In this study, we present the cryo-EM structures of two thermostable multimeric enzymes that have different point-symmetry groups; namely SOR from Acidianus ambivalens and LS from Aquifex aeolicus. The reported cryo-EM structures of the two enzymes including their active sites correlate very well with the x-ray crystal structures. Due to their thermostability and relatively easy purification scheme, both SOR and LS can serve as a model for the catalytic and structural characterization of biocatalysts as well as a benchmark for cryo-EM sample preparation, optimization of the acquisition parameters and 3D reconstruction.

LS from the hyperthermophilic bacterium Aquifex aeolicus living in hot springs of up to 90°C is extremely thermostable with a 119.9°C melting temperature, which is ~27°C higher than that of the next thermostable LS from B. subtilis. LS catalyzes the formation of 6,7-dimethyl-8-ribityllumazine by condensation of 5-amino-6-(D-ribitylamino)uracil with 3,4-dihydroxy-2-butanone 4-phosphate. LS consists of 60 identical subunits that form a capsid of icosahedral 532 symmetry with an outer diameter of 154 Å and inner compartment diameter of 80 Å. Further processing and refinement resulted in a cryo-EM map at a global 2.33 Å resolution as depicted in the FSC plot. The RMSD of both structures is 0.174 Å for the 154 Cα atoms. The LS monomer is composed of a central four-stranded β-sheet flanked on one side by two α helices and on the other side by three α helices. There is a channel in the center of the pentamer formed by an α helix (α3) and its four symmetry-related neighbors, with a diameter of about 9 Å, where most of the amino acids inside the channel are hydrophilic. The residue R40L forms salt-bridges with residues D36L, E145x and a hydrogen bridge with residue G6x, while the residue R21F forms an ion-pair with E5x which itself interacts with R52F. The R108x residue interacts with R154x within the same chain and forms an ionic contact with E65m from another chain, while R68m forms a main-chain contact to the oxygen in G64m.

>MQIYEGKLTAEGLRFGIVASRFNHALVDRLVEGAIDCIVRHGGREEDITLVRVPGSWEIPVAAGELARKEDIDAVIAIGVLIRGATPHFDYIASEVSKGLANLSLELRKPITFGVITADTLEQAIERAGTKHGNKGWEAALSAIEMANLFKSLR[60x]> MGVVEEAHNVKVIGSGEATIVLGHGFGTDQSVWKHLVPHLVDDYRVVLYDNMGAGTTNPDYFDFDRYSNLEGYSFDLIA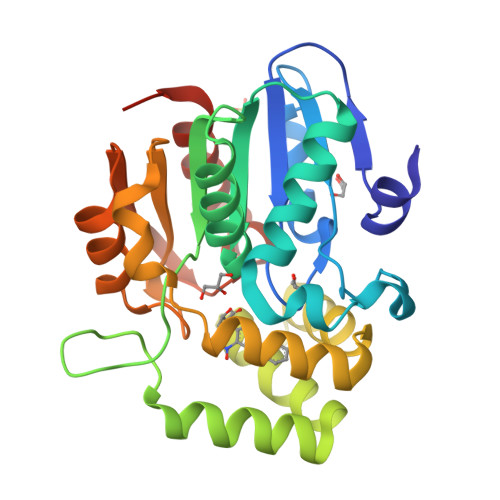ILEDLKIESCIFVGHSVSAMIGVLASLNRPDLFSKIVMISASPRYVNDVDYQGGFEQEDLNQLFEAIRSNYKAWCLGFAPLAVGGDMDSIAVQEFSRTLFNMRPDIALSVGQTIFQSDMRQILPFVTVPCHILQSVKDLAVPVVVSEYLHANLGCESVVEVIPSDGHLPQLSSPDSVIPVILRHIRNDIAMENLYFQ WD40 proteins are a subfamily of propeller proteins with no intrinsic enzymatic activity, but their stable, modular architecture and versatile surface have allowed evolution to adapt them to many vital roles. By computationally reverse-engineering the duplication, fusion and diversification events in the evolutionary history of a WD40 protein, a perfectly symmetrical homologue called Tako8 was made. A different computational approach was employed to redesign Tako8 to create Ika8, a fourfold-symmetrical protein in which neighbouring blades carry compensating charges. Tako and Ika are the first successfully designed eight-bladed WD40-repeat proteins for which structures have been confirmed crystallographically.

In contrast to Tako, Ika expressed well as a polypeptide with two, four or eight blades. Ika2 and Ika4, carrying two or four blades per subunit, respectively, were found to assemble spontaneously into a complete eight-bladed ring in solution. Ika8 produced two crystal forms in space group P63, with one or three copies in the asymmetric unit. Ika4, however, crystallized in space group P212121. In one crystal form of Ika8 this axis is crystallographic, but in the other (and in the Ika4 crystals) it is noncrystallographic. In all crystal forms, the Ika proteins assemble as trimers which stack on top of each other into pillars. Unlike in the Tako8 protein, the conserved inter­actions stabilizing the crystal assembly involve hydrogen bonds between the outer rims of neighbouring molecules, while the interactions at the top face are mediated by water molecules and are not conserved. In comparison, only the alternating repeats of the Ika proteins can be superposed, in contrast to the template structure where the overlap of the individual blades is much poorer. The melting/denaturation curves show that the Ika proteins are more stable than Tako8, especially under low-salt conditions.

>GSHMGQELVSLEGHQSAITALAFSKNIVVSGAADGTIKVWDILTGQLLRDHDGHQSEVTALQFKDNIVVSGAKDGTVKVWYIGTGQELVSLEGHQSAITALAFSKNIVVSGAADGTIKVWDILTGQLLRDHDGHQSEVTALQFKDNIVVSGAKDGTVKVWYIGT[12x]> MDYKDDDDKGDHNHRHKHGDPHMSEKRSLPMVDVKIDDEDTPQLEKKIKRQSIDHGVGSEPVSTIEIIPSDSFRKYNSQGFKAKDTDLMGTQLESTFEQELSQMEHDMADQEEHDLSSFERKKLPTDFDPSLYDISFQQIDAEQSVLNGIKDENTSTVVRFFGVTSEGHSVLCNVTGFKNYLYVPAPNSSDANDQEQINKFVHYLNETFDHAIDSIEVVSKQSIWGYSGDTKLPFWKIYVTYPHMVNKLRTAFERGHLSFNSWFSNGTTTYDNIAYTLRLMVDCGIVGMSWITLPKGKYSMIEPNNRVSSCQLEVSINYRNLIAHPAEGDWSHTAPLRIMSFDIECAGRIGVFPEPEYDPVIQIANVVSIAGAKKPFIRNVFTLNTCSPITGSMIFSHATEEEMLSNWRNFIIKVDPDVIIGYNTTNFDIPYLLNRAKALKVNDFPYFGRLKTVKQEIKESVFSSKAYGTRETKNVNIDGRLQLDLLQFIQREYKLRSYTLNAVSAHFLGEQKEDVHYSIISDLQNGDSETRRRLAVYCLKDAYLPLRLMEKLMALVNYTEMARVTGVPFSYLLARGQQIKVVSQLFRKCLEIDTVIPNMQSQASDDQYEGATVIEPIRGYYDVP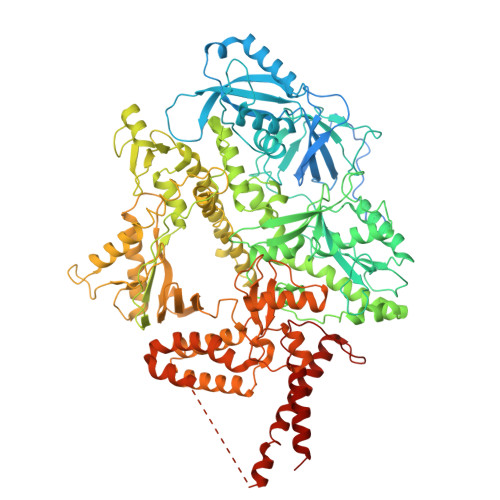IATLDFNSLYPSIMMAHNLCYTTLCNKATVERLNLKIDEDYVITPNGDYFVTTKRRRGILPIILDELISARKRAKKDLRDEKDPFKRDVLNGRQLALKISANSVYGFTGATVGKLPCLAISSSVTAYGRTMILKTKTAVQEKYCIKNGYKHDAVVVYGDTDSVMVKFGTTDLKEAMDLGTEAAKYVSTLFKHPINLEFEKAYFPYLLINKKRYAGLFWTNPDKFDKLDQKGLASVRRDSCSLVSIVMNKVLKKILIERNVDGALAFVRETINDILHNRVDISKLIISKTLAPNYTNPQPHAVLAERMKRREGVGPNVGDRVDYVIIGGNDKLYNRAEDPLFVLENNIQVDSRYYLTNQLQNPIISIVAPIIGDKQANGMFVVKSIKINTGSQKGGLMSFIKKVEACKSCKGPLRKGEGPLCSNCLARSGELYIKALYDVRDLEEKYSRLWTQCQRCAGNLHSEVLCSNKNCDIFYMRVKVKKELQEKVEQLSKW Here we report that three evolutionarily-distinct BioH isoenzymes (BioH1 to BioH3) are programmed in biotin synthesis of Mycobacterium smegmatis. The BioC-aided methylation enables the resultant malonyl-ACP (CoA) methyl ester to undergo two reiterations of FAS II cycles, generating methyl pimeloyl-ACP thioester that is subsequently hydrolyzed by the promiscuous esterase BioH to give pimeloyl-ACP (pim-ACP or C7-ACP), a precursor for biotin synthesis. The enzymatic activity in vitro combined with biotin bioassay in vivo reveals that BioH2 and BioH3 are capable of removing methyl moiety from pimeloyl-ACP methyl ester to give pimeloyl-ACP, a cognate precursor for biotin synthesis. As a member of the α/β-hydrolase (i.e., esterase) family, they adopt an identical pattern of domain organization, i.e., N-terminal lid domain connected with a core domain at C-terminus.

The crystals of BioH3 were grown using the sitting-drop vapor diffusion method and diffracted up to 2.27-Å resolution. The crystal belongs to the P21 space group, and contains six protein molecules per asymmetric unit (ASU). The two BioH3 monomers contact each other via two interfaces (Interface I & Interface II), giving a 2-fold axis-centering dimeric architecture. The fact that total buried surface area of the two interfaces is over 1760 Å2 underlined the stable existence of BioH3 dimer. First, its core domain is of α/β-fold in nature, comprising of six parallel β-strands (β1–4 and β7–8), five α-helices (α1–3 and α10–11) and a short α9 turn. In contrast to its core domain, the lid domain of BioH3 is pretty unique. Apart from α-helices, the lid domain of BioH3 also contains two β-strands (β5–6) and several connecting linkers. However, crystal structure of BioH3 illustrated that only two predicted residues (S103 and H265) are localized in the catalytic triad. Instead of D248 predicted by sequence alignment, the residue D232 participates in the formation of catalytic triad. Similar to the Shigella BioH with known complex structure, the PEG-loading cavity of BioH3 are mainly formed by the side chains of hydrophobic residues (e.g., W18, F137, and F183) from its core domain.

>[6x]MNDSRNSGTLAVLVHGAWHSSLHWAAAQRGLARRGVASIAVDLPGHGLDAPVPSGYLTAGQPGLETEKSALADITMDDLADAVVDALAEVRSRFARVLLVAHSAGGGPASLAAEKAPELVDHLVYLAAFVPAARPRFTDYINAPENADVVALPIFSDPANLGAHRLNPLSSDAIEVDAIRRAFLTDMPPDAPEGWRHLLHPDEPYASLSAPVPVTPRRWGRIPRTYIRLDGDRALAPTTQNLMIAEADRLTPDNPFGVRSLPGDHSPMVHRPGELADLLAGI N,N'-DI-1,2,3,4-TETRAHYDROACRIDIN-9-YLPENTANE-1,5-DIAMINE | C31 H36 N4 | 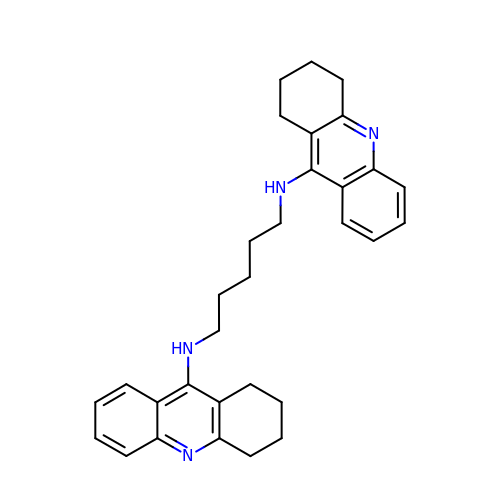NECDJQNRWSICKG-UHFFFAOYSA-N>AKPCTVSTTNATVDLGDLYSFSLMSAGAASAWHDVALELTNCPVGTSRVTA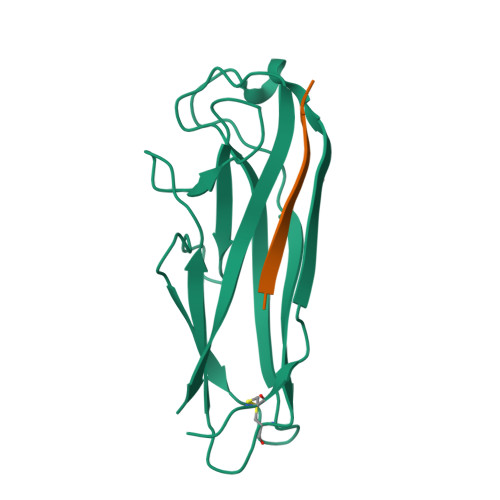SFSGAADSTGYYKNQGTAQNIQLELQDDSGNTLNTGATKTVQVDDSSQSAHFPLQVRALTVNGGATQGTIEAVISITYTYS[2x];>SRIRIRGYVR[2x]>MKRQGKRPSKNLKARCSRKALHVNFKDMGWDDWIIAPLEYEAFHCEGLCEFPLRSHLEPTNHAVIQTLMNSMDPESTPPTCCVPTRLSPISILFIDSANNVVKKDYEDMVVESCGCR[2x];>[2x]ETGQCRIQKCTTDFVSLTSHLNSAVDGFDSEFCKALRAYAGC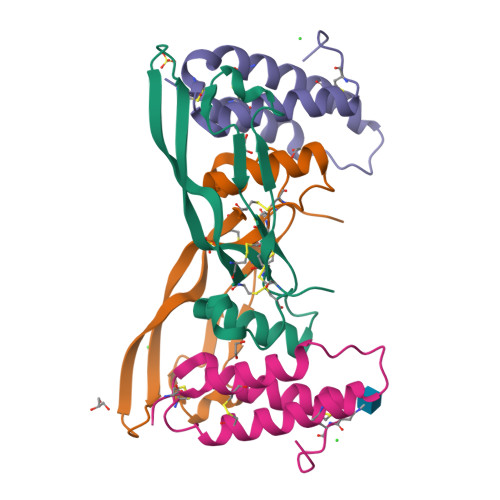TQRTSKACRGNLVYHSAVLGISDLMSQRNCSKDGPTSSTNPEVTHGTKHHHHHH> MSALCDPPGAPGPPGPAPATHGPAPLSAQELSQEIKAFLTGVDPILGHQLSAREHARCGLLLLRSLPPARAAVLDHLRGVFDESVRAHLAALDETPVAGPPHLRPPPPSHVPAGGPGLEDVVQEVQQVLSEFIRANPKAWAPVISAWSIDLMGQLSSTYSGQHQRVPHATGALNELLQLWMGCRATRTLMDIYVQCLSALIGSCPDACVDALLDTSVQHSPHFDWVVAHIGSSFPGTIISRVLSCGLKDFCVHGGAGGGAGSSGGS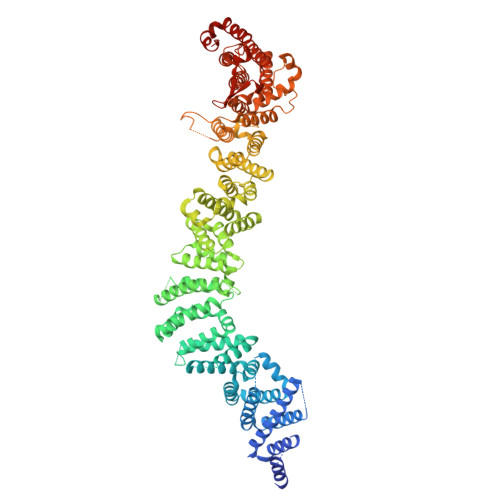SSQTPSTDPFPGSPAIPAEKRVPKIASVVGILGHLASRHGDSIRRELLRMFHDSLAGGSGGRSGDPSLQATVPFLLQLAVMSPALLGTVSGELVDCLKPPAVLSQLQQHLQGFPREELDNMLNLAVHLVSQASGAGAYRLLQFLVDTAMPASVITTQGLAVPDTVREACDRLIQLLLLHLQKLVHHRGGSPGEGVLGPPPPPRLVPFLDALKNHVGELCGETLRLERKRFLWQHQLLGLLSVYTRPSCGPEALGHLLSRARSPEELSLATQLYAGLVVSLSGLLPLAFRSCLARVHAGTLQPPFTARFLRNLALLVGWEQQGGEGPAALGAHFGESASAHLSDLAPLLLHPEEEVAEAAASLLAICPFPSEALSPSQLLGLVRAGVHRFFASLRLHGPPGVASACQLLTRLSQTSPAGLKAVLQLLVEGALHRGNTELFGGQVDGDNETLSVVSASLASASLLDTNRRHTAAVPGPGGIWSVFHAGVIGRGLKPPKFVQSRNQQEVIYNTQSLLSLLVHCCSAPGGTECGECWGAPILSPEAAKAVAVTLVESVCPDAAGAELAWPPEEHARATVERDLRIGRRFREQPLLFELLKLVAAAPPALCYCSVLLRGLLAALLGHWEASRHPDTTHSPWHLEASCTLVAVMAEGSLLPPALGNMHEVFSQLAPFEVRLLLLSVWGFLREHGPLPQKFIFQSERGRFIRDFSREGGGEGGPHLAVLHSVLHRNIDRLGLFSGRFQAPSPSTLLRQGT Trypanosoma brucei is a unicellular, protozoan parasite and the causative agent of Human African Trypanosomiasis (sleeping sickness). Here, we report that acetyl-lysine (AcK) recognizing bromodomain proteins maintain the BF cell fate in trypanosomes. The T. brucei genome contains five genes with predicted bromodomains, and we hypothesized that these proteins may play similar roles in maintaining the parasites in their BF and preventing differentiation to the PF. Consistent with its more widespread genomic localization, knockdown of Bdf3 increased transcription for more of the VSGs in the genome than was the case for Bdf2. These results imply that while both proteins maintain monoallelic expression of VSG genes, Bdf2 has a more specialized role in maintaining silencing at ESs.

Using the recombinantly expressed and purified bromodomains from T. brucei Bdf2 and Bdf3 (Tb927.10.7420, Tb927.11.10070, respectively), we performed isothermal titration calorimetry experiments and confirmed direct and specific binding of I-BET151 to their AcK recognition sites, as mutation of two conserved residues in the AcK sites abolished interaction with the inhibitor. To provide a blueprint towards designing high-affinity trypanosome-specific bromodomain inhibitors, we determined the crystal structure of the Bdf2 bromodomain in complex with I-BET151 at 1.25Å resolution. The overall structure adopts the canonical bromodomain fold comprising four α-helices linked by variable loop regions that form the ligand binding site. Unexpectedly, but consistent with the reduced affinity, the ligand is flipped by roughly 180° with respect to the human BRD4-BD1-I-BET151 complex and cannot adopt its classical binding mode. In Bdf2, the dimethylisoxazole ring is solvent-exposed, while recognition of the conserved Asn takes place through a bidentate hydrogen bond to the imidazolone moiety. The new orientation is probably due to a clash of the pendent pyridine ring with the large trypanosome gatekeeper residue Trp92, which dominates ligand recognition through parallel π–π stacking and which is not found in any of the 61 human bromodomains at this position. The flipped binding mode is further enforced by the narrow AcK binding slot that cannot accommodate the energetically favorable twist of the dimethylisoxazole with respect to the quinoline ring. Notably, the pyridine moiety forces the imidazolone to sit high up in the AcK binding pocket, resulting in an imperfect fit with a gap at the bottom of the pocket that is filled by an additional, unconserved water molecule (Wat1). However, the negative electrostatic surface potential of Bdf2 markedly differs from the slightly positively charged BRD9 pocket, highlighting the distinct character of the Bdf2 AcK binding site, a prerequisite for developing a trypanosome-specific drug.

>GPHMSFNKNGCLVFVSRLWDLDKLGMFHHPVSAEELPDYHTVIKRPVDLSSIRDGIEKGTYATDVDVQNDVARMITNALEYNAKGSTWYQEAMSFRKTYLDLARQSGLVVDDDEAYIPS[2x]> GSHMAFTPFPPRQPTASARLPLTLMTLDDWALATITGADSEKYMQGQVTADVSQMAEDQHLLAAHCDAKGKMWSNLRLFRDGDGFAWIE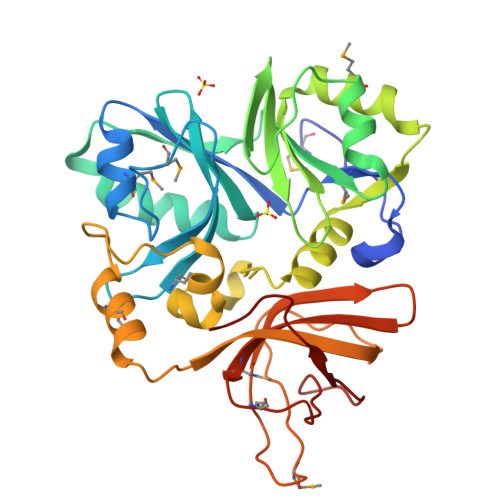RRSVREPQLTELKKYAVFSKVTIAPDDERVLLGVAGFQARAALANLFSELPSKEKQVVKEGATTLLWFEHPAERFLIVTDEATANMLTDKLRGEAELNNSQQWLALNIEAGFPVIDAANSGQFIPQATNLQALGGISFKKGCYTGQEMVARAKFRGANKRALWLLAGSASRLPEAGEDLELKMGENWRRTGTVLAAVKLEDGQVVVQVVMNNDMEPDSIFRVRDDANTLHIEPLPYSLE>MPRKKDQVTKNDDGNQTSDVQTQDFKTAVQPDTNTAQLIKTYSNPKQRGDKGEIIYDGGLSSKLADVVDKTTEPHNADGAVKDGRIAPVKLDLEKQKLDKLKLFETSPFDPLTIKNNQDVVDKLYATQSSSIQEVVPTKTFATELQFGVTSEDMAKIYGAVAAVSKNVNSSVTYEVKRGTHELIKVPTIPHNLVLIQSDNGKHALIKEDLGQWPVETGISLVNQAGVFAVQLANKLGIDKPFVLDAGSNYFTDTSFIDTRKYCTDGLSPREIQKALNRQRAYYDRPELTISENKTLLSQSIIYPDADGNDVSIIFSGAMSHAIFTYAQSQWNKNIIKLDDYIREITLTVPKQYRPRRFKEIEHTHGYVYRELNQGSLLPLVDANLKESSSYYFKKLMSSISNVPVDARTLQSATAALAADTGQAVNRAQHVSMLTNRLTTANAPTVRAITVLTCMFKQFRIGMTYALDPNIMDVAAATCMLLFRPAQSISDEQYRYCLQTMAVFLTNTTYDIVNNDTIDVLKMKLRNQGWPFVERYNAVEIDMSVEPLRSPGQVGRYYNPFNIDPLTKKHVEDRLEEFINQVQVGRFRNASGNAVGTTLAAFLRACRDKTSANWRGYSVLVSRYRSLIPNELFESLRNISGEYNINPQDEHSFFFALAQINADDEFIGAIDKESAEYLDEYATLARDISNSLTLVKAAFGPLERTSGSIINHANNLNKVINHVFADKPLISETMLKILTIDGTTGKDGYRNWLDKLVGHNYPVYVEPVVNIMNFISARFVADSSYFGYTNEIMIMPNHINVPVDDRFGFRDSPFCTSLPRTIMGNDVRRISYNVFSMMEDIDDVISEGFILYDAYFNFSYDIMTTDGVTRLKEDILIVTDTGNDIKPIHFYIYFENRNDKKLRYESKMNVSYRLYIKTPACLLPLSDYMRAQHDYVSPSSSRVYIKDPAVVYTRS[2x];>MANRATSAFLDNPHPVGVNYVDEGSRQFVAVAELLASKLIDSSRESDESNSDVPFVQAYSKFADDNPRHLRVKTGGKMANALTNVIRSYYSINAPAIVPQVEIDRLASKATVSGDMYNSYAIFNSVPIVEVLSPARTTVSIVGSDRADVTMLNTGAGAANITFNFGQIAETVILKGSVPFQLARLNQPMPAARFTYKLRPLDGPFIVVLPVGNPLVISATAATRIQVPLAFNKALVESGFQTAMNDGLFDIQNVNYYSSFDEFIISQYHAQDGINRVSTCVILGLALQAYDQMRRALPVRRV[13x];>MDVLSKGSLKELLAHLEKTPLEEAISYRIGTVPYQNVLISRNEYYNQLYPDTTSLIDGVSREGQRNVNGLIMSIISYVVSGSGHYIPNIGFMLLRRSILDILTKHDTGLVTNNLNYGIIARNLTVSKMNCEQRKRMLICFKLLAYKDGNQNDYEIYLNQNIPLKQIAPNFIPGDMRTVIHNQDQLAIVGIPAYRLTQSTELSIRDDNAKSYKLGYVDWYNSNSFLRERSEFNLIRLKDRDTKYGKLNGW[2x];>MAWVTQAYSSGLSQNSIISLTGNDRTVADGTFNSMIMPRAVIANEREHFMKTRIDKIEHDLNRSAKQEMMDRQSLAEDYNALNLAVGQEIKLDIATQHQLNRLGSAMYKADHERETELTDLINRIRENEVTVNGILENQKAITAAERADLLLEVVASTAKSVSAAGRAAADGSGVVPVFGPSVANGIKVGIDIADSVAEAAIAVKESGIITQLNDVYHAFQSVHVAPNDVIKPAAVVAGTSTELIGNLQAIYSRLRSHSDIGFKKATVGDVIPNSYMIKPVNSTEYASWQLYVIHPVQGSLGLVVQLMGDALTYNVFAQYGNTSASEFGKTVLTGGATNTALEGTKVKFQTKVTAQQALALTMALKDAASMLSQGELIGYFEQYINLALEPDNLSLQDNMHKYHHLLTSQNSPIDWNYHDEEMHKWLDSRKTTNYDAMQKKDGTVIADIHIPKVFNDLRNTTLHCKLEGKQTIAGYTVYEYLIGPWAHYGDIDYSVVVDTLNEETKWYCEVIGIDGHLLIEKSVQHKPEKILELTVNDSGVTSFNGRNHDRLKLKVYVKDSLSVKVFRNWIGINAPRVKTKMFNDHIGVKYDYSHFDKNISPAHLTLTDLGWHTWDQYNAGNWTNIKP[3x];>MLSETELRALKKLSTTTSRVVGDSTLALPSNVKLSKGEVEKIAVTKKEMFDELAQCNLPTIELITREHTFNGDVIRFAAWLFLMNGQKLMIANNVAVRMGMQYATNLAGNNVKITYVTSNNVVKLGHIAAGVLANPYSNKGSGLFITYEYNLISNLIETGKVCVLFITSLSTTASSTNSFAYSTCSVPIENWDFNMIKLTAETSCASLTAMTNLVNSLVPGERTRPVGLYVDIPGVTVTTSASSGSLPLTTIPAVTPLIFSAYTKQVEEVGVINTLYALSYLP[3x]

Banna virus (BAV) is the prototype Seadornavirus, a class of reoviruses for which there has been little structural study. Here, we report atomic cryo-EM structures of three states of BAV virions—surrounded by 120 spikes (full virions), 60 spikes (partial virions), or no spikes (cores). In the full and partial BAV virions, genomic dsRNA segments and a number of RNA-dependent RNA polymerases (RdRps, VP1) are packaged in a double-layered icosahedral capsid consisting of three proteins (VP2, VP8, and VP10). The spikes protruding from the outer capsid shell are heterohexamers composed of a VP4 trimer capped by a VP9 trimer.

Visual inspection and 2D class averaging of purified BAV YN15-126-01 virions on cryo-EM micrographs revealed two types of virions: one surrounded by more spikes on the viral surface (hereafter referred to as full particles), and the other with sparser spiky density (partial particles). The ratio of full to partial particles was approximately 3:1. Icosahedral reconstructions of full and partial BAV particles (at ~5.7 Å resolution) revealed that they share overall structural features except for the different number of spikes on the virus surface. In the full BAV virions, there are 60 spikes sitting on VP10A and VP10B, respectively, while in the partial virions, there are only 60 spikes on VP10A. The binding affinity of spikes at the two channels appears different, resulting in detachment of half the spikes when the partial particles form. At physiological pH, VP4 (pI = 5.9, negatively charged) would electrostatically interact with the basic VP10 protein (pI = 9.0), suggesting that electrostatic interactions between the VP4 trimer and VP10 may play an important role in association of spikes on the virus surface. Binding of VP4 trimers also results in a total ~1800 Å2 of buried surface area on VP8 molecules surrounding VP10A, which is ~10% more than for VP8 surrounding VP10B ( ~ 1600 Å2), likely contributing to different affinity of VP4 trimers for the outer capsid shell in the full BAV particles. In the cryo-EM structure at overall 6 Å-resolution based on ~1400 acidified virus particles, 16-nm rod-shaped projections (the density of VP4 at ~15 Å local resolution) arise only from VP10A at the type II channel, suggesting that the specific shedding of spikes that occurs on partial particles may be required to form this acidified conformation. BAV entry into the cell is a highly ordered process with stepwise detachment of viral spikes, as reflected by the variation in spike arrangement on full particles (120 spikes containing VP4 and VP9), partial particles (60 spikes containing VP4 and VP9), acidified particles (60 spikes containing VP4), and core particles (no spikes).> MAHHHHHHHHHHSGRELQPPEASIAVVSIPRQLPGSHSEAGVQGLSAGDDSETGSDCVTQAGLQLLASSDPPALASKNAEVTVETGFHHVSQADIEFLTSIDPTASASGSAGITGTMSQDTEVDMKEVELNELEPEKQPMNAASGAAMSLAGAEKNGLVKIKVAEDEAEAAAAAKFTGLSKEELLKVAGSPGWVRTRWALLLLFWLGWLGMLAGAVVIIVRAPRCRELPAQKWWHTGALYRIGDLQAFQGHGAGNLAGLKGRLDYLSSLKVKGLVLGPIHKNQKDDVAQTDLLQIDPNFGSKEDFDSLLQSAKKKSIRVILDLTPNYRGENSWFSTQVDTVATKVKDALEFWLQAGVDGFQVRDIENLKDASSFLAEWQNITKGFSEDRLLIAGTNSSDLQQILSLLESNKDLLLTSSYLSDSGSTGEHTKSLVTQYLNATGNRWCSWSLSQARLLTSFLPAQLLRLYQLMLFTLPGTPVFSYGDEIGLDAAALPGQPMEAPVMLWDESSFPDIPGAVSANMTVKGQSEDPGSLLSLFRRLSDQRSKERSLLHGDFHAFSAGPGLFSYIRHWDQNERFLVVLNFGDVGLSAGLQASDLPASASLPAKADLLLSTQPGREEGSPLELERLKLEPHEGLLLRFPYAALE;> MADYKDDDDKSGPDEVDASGRVRKPVVSTISKGGYLQGNVNGRLPSLGNKEPPGQEKVQLKRKVTLLRGVSIIIGTIIGAGIFISPKGVLQNTGSVGMSLTIWTVCGVLSLFGALSYAELGTTIKKSGGHYTYILEVFGPLPAFVRVWVELLIIRPAATAVISLAFGRYILEPFFIQCEIPELAIKLITAVGITVVMVLNSMSVSWSARIQIFLTFCKLTAILIIIVPGVMQLIKGQTQNFKDAFSGRDSSITRLPLAFYYGMYAYAGWFYLNFVTEEVENPEKTIPLAICISMAIVTIGYVLTNVAYFTTINAEELLLSNAVAVTFSERLLGNFSLAVPIFVALSCFGSMNGGVFAVSRLFYVASREGHLPEILS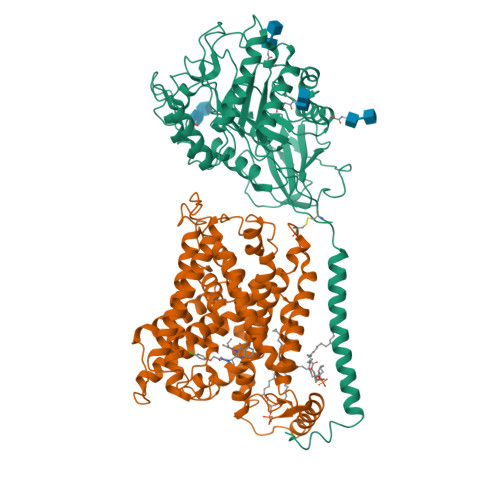MIHVRKHTPLPAVIVLHPLTMIMLFSGDLDSLLNFLSFARWLFIGLAVAGLIYLRYKCPDMHRPFKVPLFIPALFSFTCLFMVALSLYSDPFSTGIGFVITLTGVPAYYLFIIWDKKPRWFRIMSEKITRTLQIILEVVPEEDKL> MGPAKQYDSVECPFCDEVSKYEKLAKIGQGTFGEVFKARHRKTGQKVALKKVLMENEKEGFPITALREIKILQLLKHENVVNLIEICRTKASPYNRCKASIYLVFDFCEHDLAGLLSNVLVKFTLSEIKRVMQM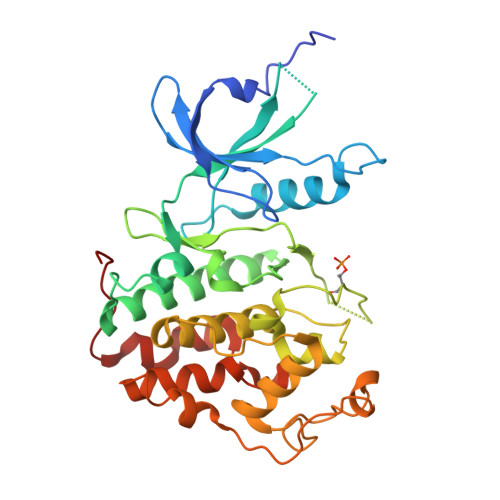LLNGLYYIHRNKILHRDMKAANVLITRDGVLKLADFGLARAFSLAKNSQPNRYTNRVVTLWYRPPELLLGERDYGPPIDLWGAGCIMAEMWTRSPIMQGNTEQHQLALISQLCGSITPEVWPNVDNYELYEKLELVKGQKRKVKDRLKAYVRDPYALDLIDKLLVLDPAQRIDSDDALNHDFFWSDPMPSDLKGMLST> SKSCDTVDLGYQCSPATSHLWGQYSPFFSLEDELSVSSKLPKDCRITLVQVLSRHGARYPTSSKSKKYKKLVTAIQANATDFKGKFAFLKTYNYTLGADDLTPFGEQQLVNSGIKFYQRYKALARSVVPFIRASGSDRVIASGEKFIEGFQQAKLADPGATNRAAPAISVIIPESETFNNTLDHGVCTKFEASQLGDEVAANFTALFAPDIRARAEKHLPGVTLTDEDVVSLMDMCSFDTVARTSDASQLSPFCQLFTHNEWKKYNYLQSLGKYYGYGAGNPLGPAQGIGFTNELIARLTRSPVQDHTSTNSTLVSNPATFPLNATMYVDFSHDNSMVSIFFA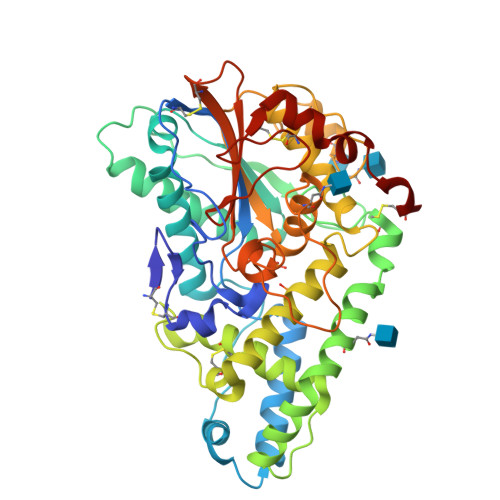LGLYNGTEPLSRTSVESAKELDGYSASWVVPFGARAYFETMQCKSEKEPLVRALINDRVVPLHGCDVDKLGRCKLNDFVKGLSWARSGGNWGECFS>[3x]PMFIVNTNV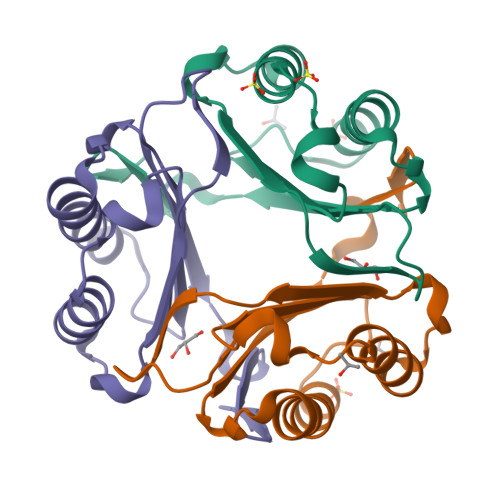PRASVPDGFLSELTQQLAQATGKPPQYIAVHVVPDQLMAFGGSSEPCALCSLHSIGKIGGAQNRSYSKLLCGLLAERLRISPDRVYINYYDMNAANVAWNNSTFA> MPTVDDILEQVGESGWFQKQAFLILCLLSAAFAPICVGIVFLGFTPDHHCQSPGVAELSQRCGWSPAEELNYTVPGLGPAGEAFLGQCRRYEVDWNQSALSCVDPLASLATNRSHLPLGPCQDGWVYDTPGSSIVTEFNLVCADSWKLDLFQSCLNAGFLFGSLGVGYFADRFGRKLCLLGTVLVNAVSGVLMAFSPNYMSMLLFRLLQGLVSKGNWMAGYTLITEFVGSGSRRTVAIMYQMAFTVGLVALTGLAYALPHWRWLQLAVSLPTFLFLLYYWCVPESPRWLLSQKRNTEAIKIMDHIAQKNGKLPPADLKMLSLEEDVTEKLSPSFADLFRTPRLRKRTFILMYLWFTDSVLYQGLILHMGATSGNLYLDFLYSALVEIPGAFIALITIDRVGRIYPMAMSNLLAGAACLVMIFISPDLHWLNIIIMCVGRMGITIAIQMICLVNAELYPTFVRNLGVMVCSSLCDIGGIITPFIVFRLREVWQALPLILFAVLGLLAAGVTLLLPETKGVALPETMKDAENLGRKAKPKENTIYLKVQTSEPSGTEDQVDPRLIDGK

The human organic cation transporter 1 (hOCT1), also known as SLC22A1, is integral to hepatic uptake of structurally diversified endogenous and exogenous organic cations, influencing both metabolism and drug pharmacokinetics. hOCT1 has been implicated in the therapeutic dynamics of many drugs, making interactions with hOCT1 a key consideration in novel drug development and drug–drug interactions. As part of the major facilitator superfamily (MFS), hOCT1 operates on an alternating access mechanism, allowing substrate-binding sites to be exposed alternately to either side of the membrane via transporter conformational changes. Each hOCT1 transport cycle involves transitioning from the outward open to the outward occluded, then inward occluded, and finally the inward open states. The protein can be divided into several different regions, with the N-terminal domain (NTD) comprising transmembrane helices 1–6 (TMs 1–6), and the C-terminal domain (CTD), consisting of transmembrane segments 7–12 (TMs 7-12).

In the case of hOCT1-metformin in DDM micelles, we successfully delineated structures in three conformations: outward open (hOCT1-M1), outward occluded (hOCT1-M2), and inward occluded (hOCT1-M3), at resolutions ranging from 3.8 to 4.1 Å. In its outward open state, the hOCT1 metformin-binding site exposed extracellularly. The channel connecting the extracellular environment to the binding site is negatively charged, potentially enhancing selectivity for positively charged organic cation substrates. Metformin is situated within the central cavity, forming cation-π interaction with Y361 on TM7, with Q362 also likely contributing to substrate binding. Consistent with the findings from 2D classification, the ICH domain densities are exclusive to outward facing conformations, irrespective of hOCT1 complex formation with either metformin or spironolactone. The shift from the outward open to the occluded state is characterized by the movement of the extracellular termini of the CTD helices, with the intracellular portions of these helices exhibiting minimal displacement.>[2x]NVGKKYFMSS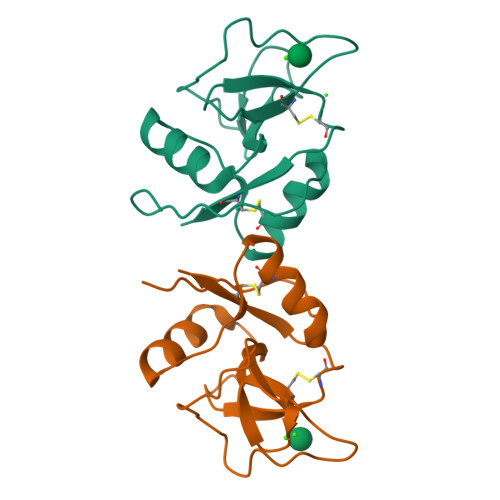VRRMPLNRAKALCSELQGTVATPRNAEENRAIQNVAKDVAFLGITDQRTENVFEDLTGNRVRYTNWNEGEPNNVGSGENCVVLLTNGKWNDVPCSDSFLVVCEFS>[2x]GDDLEVGKNIDESAYSGIYENNAYLRDGKSNLVSKVVELHGETYATTVKMGLSKTPNTATSAKVKIDAAYLETYNKAHNTDFALYPQDLVTFANEGILTVNANTKSAEVEMTIRAGEGLQEDKTYAIPVAISDQSSDITIKDEDAKHCIYLVKDMRNAGDAYKGEGVMQGYLFFEVNDVNPLNTLSFQLENGKLLWDVVVLFAANINYDAEAGRPRVQCNPNVQY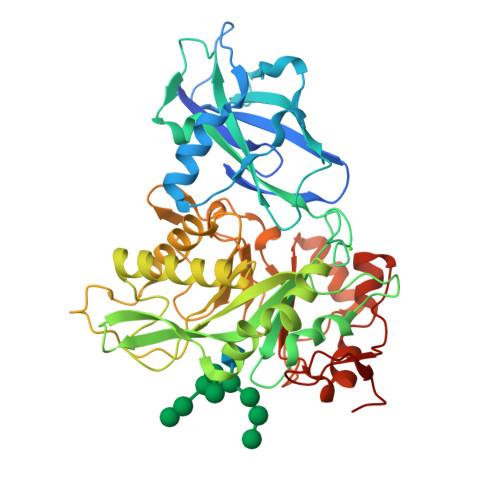LLDNNETLLQPLRRRGVKVLLGLLGNHDITGLAQLSEQGAKDFAREVAQYCKAYNLDGVNYDDEYSNSPDLSNPSLTNPSTAAAARLCYETKQAMPDKLVTVFDWGQMYGVATVDGVDAKEWIDIVVANYGSAAYPIGQMTKKQCSGISMEFNLGGGGSLSASKAQSMIDGGYGWFMGFAPSPAKYGSVFSRLQGGGEVLYGSNVAAPTIFYKKNDPTPYKYPDDL>MARRLPKPTLQGRLEADFPDSPLLPKFQELNQNNLPNDVFREAQRSYLVFLTSQFCYEEYVQRTFGVPRRQRAIDKRQRASVAGAGAHAHLGGSSATPVQQAQAAASAGTGALASSAPSTAVAQSATPSVSSSISSLRAATSGATAAASAAAAVDTGSGGGGQPHDTAPRGARKKQ[4x];>MKVQGSVDRRRLQRRIAGLLPPPARRLNISRGSEFTRDVRGLVEEHAQASSLSAAAVWRAGLLAPGEVAVAGGGSGGGSFSWSGWRPPVFGDFLIHASSFNNAEATGTPLFQFKQSDPFSGVDAVFTPLSLFILMNHGRGVAARVEAGGGLTRMANLLYDSPATLADLVPDFGRLVADRRFHNFITPVGPLVENIKSTYLNKITTVVHGPVVSKAIPRSTVKVTVPQEAFVDLDAWLSGGAGGGGGVCFVGGLGLQPCPADARLYVALTYEEAGPRFTFFQSSRGHCQIMNILRIYYSPSIMHRYAVVQPLHIEELTFGAVACLGTFSATDGWRRSAFNYRGSSLPVVEIDSFYSNVSDWEVIL[2x];>[4x]MDLKVVVSLSSRLYTDEIAKMQQRIGCILPLASTHGTQNVQGLGLGQVYSLETVPDYVSMYNYLSDCTLAVLDEVSVDSLILTKIVPGQTYAIKNKYQPFFQWHGTGSLSVMPPVFGREHATVKLESNDVDIVFPMVLPTPIAEEVLQKILLFNVYSRVVMQAPGNADMLDVHMHLGSVSYLGHHYELALPEVPGPLGLALLDNLSLYFCIMVTLLPRASMRLVRGLIRHEHHDLLNLFQEMVPDEIARIDLDDLSVADDLSRMRVMMTYLQSLASLFNLGPRLATAAYSQETLTATCWLR;>[2x]MSNGDWGQSQRTRGTGPVRGIRTMDVNAPGGGSGGSALRILGTASCNQAHCKFGRFAGIQCVSNCVLYLVKSFLAGRPLTSRPELDEVLDEGARLDALMRQSGILKGHEMAQLTDVPSSVVLRGGGRVHIYRSAEIFGLVLFPAQIANSAVVQSLAEVLHGSYNGVAQFILYICDIYAGAIIIETDGSFYLFDPHCQKDAAPGTPAHVRVSTYAHDILQYVGAPGAQYTCVHLYFLPEAFETEDPRIFMLEHYGVYDFYEANGSGFDLVGPELVSSDGEAAGTPGADSSPPVMLPFERRIIPYNLRPLPSRSFTSDSFPAARYSPAKTNSPPSSPASAAPASAAPASAAPASAAPASAAPASAAPASAAPASAAPASSPPLFIPIPGLGHTPGVPAPSTPPRASSGAAPQTPKRKKGLGKDSPHKKPTSGRRLPLSSTTDTEDDQLPRTHVPPHRPPSAARLPPPVIPIPHQSPPASPTPHPAPVSTIAPSVTPSPRLPLQIPIPLPQAAPSNPKIPLTTPSPSPTAAAAPTTTTLSPPPTQQQPPQSAAPAPSPLLPQQQPTPSAAPAPSPLLPQQQPPPSAARAPSPLPPQQQPLPSATPAPPPAQQLPPSATTLEPEKNHPPAADRAGTEISPSPPFGQQPSFGDDASGGSGLVRYLSDLEEPFLSMSDSEEAESDLASDIPTTEDEDMFEDEVFSNSLESGSSAPTSPITLDTARSQYYQTTFDIETPEMDFVPLESNIARIAGHTYQEQAIVYDPASNREVPEADALSMIDYLLVTVVLEQGLIRSRDRSSVLNLLEFLKDWSGHLQVPTLDLEQLLTSELNIQNLANMLSENKGRAGEFHKHLAAKLEACLPSLATKDAVRVDAGAKMLAEIPQLAESDDGKFDLEAARRRLTDLLSGGDQEAGEGGGEPEDNSIYRGPHVDVPLVLDDESWKRLLSLAEAARTAVARQQAGVDEEDVRFLALLTAIEYGAPPAASVPPFVHNVAVRSKNAALHVRRCTADIRDKVASAASDYLSYLEDPSLPTVMDFDDLLTHLRHTCQIIASLPLLNIRYTSIEWDYRELLYLGTALSDMSGIPWPLERVEEDDPSIAPLPEFETVAKKQKELETTRENEKRLRTILDDIEAMLGLAGVASAPGAPISPASPSATPANHDNPEATPPLADTAALTIPVIEKYIANAGSIVGAAKNPTYIRLRDTIQQIVRSKKYLMNILKSITFYTIDNYIASFEESIDHLYRDLPVLDPEVQDGIDRILDPMVSEALHTFEMGNRLTLEPARLVALQNFATHSTLKETAAAVNLLPGLLAVYDATITGQAPEDALRLLSGLQNQLSQTLIPGKLKKRFLSYLQKLKNNNNDQLRQKEVQAWRLEAEGFKPATEEQLEAFLDTAPNKELKRQYEKKLRQLMETGRKEKEKLREQEDKERQERRAREANEAWARIRKALGARPEPAPTSPDDWNTLLASLLPDNTDSAAAAAAAVARNTDILDSLTQILAAMLLGITRVRRERLRSLLVDDGGAAERMEAAEPGWFTDIETGPLARLDAWPATPAATAKEGGGGRGAEEAAGALFRARTAADAIRSALAQTRQALQSPDMKSAVVNTDLEAPYAEYERGLAGLLEKRRAAEAALTAIVSEYVDRTLPEATNDPGQANLPPPPTIPQATAPPRLASDSALWPKKPQLLTRRERDDLLQATGDFFSELLTEAEAAEVRALEEQVRESQTLMAKAHEMAASTRRGFHTALEAVLSRSRDEAPDDELRSLLPSPPKAPVQAPLEAALARAAAGNGSWPYRKSLAAAKWIRGICEAVRGLSEGALALAGGAGAWLNLAAAADGEIHELTRLLEVEGMAQNSMDGMEELRLALATLDPKRVAGGKETVADWKRRLSRLEAIIQEAQEESQLQGTLQDLVTQARGHTDPRQLKIVVEAARGLALGASAGSQYALLKDKLLRYASAKQSFLAFYETAQPTVFVKHPLTNNLPLLITISAPPTGWGNGAPTRRAQFLAAAGPAKYAGTLWLETESPCDPLNPAYVSADTQEPLNYIPVYHNFLEYVMPTVLENPEAFSLTPAGRPQAIGPPQDDQERRRRTLASVASARLSAAAADSYWDTWPDVESNAGELLREYVSAPKALMEDLADNPIVAMTLLAHASLIASRNHPPYPAPATDREVILLEQREMMALLVGTHPAYAAAFLGAPSFYAGLGLVSALARDGGLGDLLSDSVLTYRLVRSPASGRGGMPSTTRGSNDGEDARRLTRHRIAGPPTGFIFFQDAWEEMDTRAALWPHPEFLGLVHNQSTARARACMLLLARRCFAPEALQQLWHSLRPLEGPVAFQDYLRDFVKQAYTRGEELPRAEGLEVPRETPSSYGTVTGRALRNLMPYGTPITGPKRGSGDTIPVSVFEAAVAAAFLGRPLTLFVSSQYLFNLKTLGQVRVVAPLLYCDGHSEPFRSLVETISLNFLQDLDGYSESFEPEMSIFARQAVWLRELLTEARAAKPKEARPPTVAILANRKNIIWKCFTYRHNLPDVQFYFNAAGASRWPTDVLNPSFYEHEDPPLPVGYQLPPNPRNVQELFSGFPPRVGHGLVSGDGFQSADNTPASSDRLQQLGGGETDQGEKGSTTAESEASGPPSPQSPLLEKVAPGRPRDWLSPTSSPRDVTVTPGLAAPITLPGPRLMARPYFGAETRASESPDRSPGSSPRPWPKDSLELLPQPAPQQPPSSPWASEQGPIVYTLSPHSTPSTASGSQKKHTIQIPGLVPSQKPSYPPSAPYKPGQSTGGIAPTPSAASLTTFGLQPQDTQASSQDPPYGHSIMQREKKQQGGREEAAEIRPSATRLPTAVGLRPRAPVVAAGAAASATPAFDPGEAPSGFPIPQAPALGSGLAAPAHTPVGALAPRPQKTQAQRPQDAAALPTPTIKAVGARPVPKATGALAAGARPRGQPTAAPPSAASPPRVSLPVRSRQQQSPAIPLPPMHSGSEPGARPEVRLSQYRHAGPQTYTVRKEAPPSAASQLPKMPKCKDSMYYPPSGSARYPAPFQALSFSQSVASPAPSSDQTTLLWNTPSVVTQFLSIEDIIREVVTGGSTSGDLVVPSGSPSSLSTAAPEQDLRYSLTLSQASRVLSRFVSQLRRKLERSTHRLIADLERLKFLYL;> MDVHIDNQVLSGLGTPLLVHLFVPDTVMAELCPNRVPNCEGAWCQTLFSDRTGLTRVCRVFAARGMLPGRPSHRGTFTSVPVYCDEGLPELYNPFHVAALRFYDEGGLVGELQIYYLSLFEGAKRALTDGHLIREASGVQESAAAMQPIPIDPGPPGGAGIEHMPVAAAQVEHPKTYDLKQILLEITQEENRGEQRLGHAGSPALCLGLRLRAGAETKAAAETSVSKHHPALENPSNIRGSAGGEGGGGRAGTGGTVGVGSGALSRVPVSFSKTRRAIRESRALVRGIAHIFSPHALYVVTYPELSAQGRLHRMTAVTHASPATDLAEVSILGAPEREFRFLISVALRISASFREKLAMQAWTAQQEIPVVIPTSYSRIYKNSDLIREAFFTVQTRVSWESCWVKATISNAPKTPDACLWIDSHPLYEEGASAWGKVIDSRPPGGLVGAASQLVALGTDGHCVHLATTSDGQAFLVLPGGFVIKGQLALTPEERGYILARHGIRREQ;>MALSGHVLIDPARLPRDTGPELMWAPSLRNSLRVSPEALELAEREAERARSERWDRCAQVLKNRLLRVELDGIMRDHLARAEEIRQDLDAVVAFSDGLESMQVRSPSTGGRSAPAPPSPSPAQPFTRLTGNAQYAVSISPTDPPLMVAGSLAQTLLGNLYGNINQWVPSFGPWYRTMSANAMQRRVFPKQLRGNLNFTNSVSLKLMTEVVAVLEGTTQDFFSDVRHLPDLQAALILSVAYLLLQGGSSHQQRPLPASREELLELGPESLEKIIADLKAKSPGGNFMILTSGNKEARQSIAPLNRQAAYPPGTFADNKIYNLFVGAGLLPTTAALNVPGAAGRDRDLVYRIANQIFGEDVPPFSSHQWNLRVGLAALEALMLVYTLCETANLAEAATRRLHLSSLLPQAMQRRKPAMASAGMPGAYPVQTLFRHGELFRFIWAHYVRPTVAADPQASISSLFPGLVLLALELKLMDGQAPSHYAINLTGQKFDTLFEIINQKLLFHDPAAMLAARTQLRLAFEDGVGVALGRPSPMLAAREILERQFSASDDYDRLYFLTLGYLASPVAPS[2x];>MASNEGVENRPFPYLTVDADLLSNLRQSAAEGLFHSFDLLVGKDAREAGIKFEVLLGVYTNAIQYVRFLETALAVSCVNTEFKDLSRMIDGKIQFRISVPTIAHGDGRRPSKQRTFIVVKNCHKHHISTEMELSMLDLEILHSIPETPVEYAEYVGAVKTVASALQFGVDALERGLINTVLSVKLRHAPPMFILQTLADPTFTERGFSKTVKSDLIAMFKRHLLEHSFFLDRAENMGSGFSQYVRSRLSEMVAAVSGESVLKGVSTYTTAKGGEPVGGVFIVTDNVLRQLLTFLGEEADNQIMGPSSYASFVVRGENLVTAVSYGRVMRTFEHFMARIVDSPEKAGSTKSDLPAVAAGVEDQPRVPISAAVIKLGNHAVAVESLQKMYNDTQSPYPLNRRMQYSYYFPVGLFMPNPKYTTSAAIKMLDNPTQQLPVEAWIVNKNNLLLAFNLQNALKVLCHPRLHTPAHTLNSLNAAPAPRDRRETYSLQHRRPNHMNVLVIVDEFYDNKYAAPVTDIALKCGLPTEDFLHPSNYDLLRLELHPLYDIYIGRDAGERARHRAVHRLMVGNLPTPLAPAAFQEARGQQFETATSLAHVVDQAVIETVQDTAYDTAYPAFFYVVEAMIHGFEEKFVMNVPLVSLCINTYWERSGRLAFVNSFSMIKFICRHLGNNAISKEAYSMYRKIYGELIALEQALMRLAGSDVVGDESVGQYVCALLDPNLLPPVAYTDIFTHLLTVSDRAPQIIIGNEVYADTLAAPQFIERVGNMDEMAAQFVALYGYRVNGDHDHDFRLHLGPYVDEGHADVLEKIFYYVFLPTCTNAHMCGLGVDFQHVAQTLAYNGPAFSHHFTRDEDILDNLENGTLRDLLEISDLRPTVGMIRDLSASFMTCPTFTRAVRVSVDNDVTQQLAPNPADKRTEQTVLVNGLVAFAFSERTRAVTQCLFHAIPFHMFYGDPRVAATMHQDVATFVMRNPQQRAVEAFNRPEQLFAEYREWHRSPMGKYAAECLPSLVSISGMTAMHIKMSPMAYIAQAKLKIHPGVAMTVVRTDEILSENILFSSRASTSMFIGTPNVSRREARVDAVTFEVHHEMASIDTGLSYSSTMTPARVAAITTDMGIHTQDFFSVFPAEAFGNQQVNDYIKAKVGAQRNGTLLRDPRTYLAGMTNVNGAPGLCHGQQATCEIIVTPVTADVAYFQKSNSPRGRAACVVSCENYNQEVAEGLIYDHSRPDAAYEYRSTVNPWASQLGSLGDIMYNSSYRQTAVPGLYSPCRAFFNKEELLRNNRGLYNMVNEYSQRLGGHPATSNTEVQFVVIAGTDVFLEQPCSFLQEAFPALSASSRALIDEFMSVKQTHAPIHYGHYIIEEVAPVRRILKFGNKVVF[4x]

Epstein-Bar virus (EBV), a member of the subfamily gammaherpesviruses that also includes the Kaposi Sarcoma-associated herpesvirus (KSHV),2,3 is the first identified oncovirus. Similar to other members of the family herpesviridae, EBV has a characteristic three-layer configuration: the outer lipid bilayer envelope containing viral glycoproteins responsible for host recognizing and membrane fusion, the inner pseudo-icosahedral nucleocapsid enclosing a 172-kb double-strand DNA (dsDNA) genome and the middle pleomorphic tegument compartment fulfilled with 20–40 different viral proteins. All herpesvirus capsid shell consists of 4 abundant proteins: the major capsid proteins (MCP) constituting the basic capsid skeleton through forming 150 hexons and 11 pentons, the small capsid proteins (SCP) binding to the tops of hexon MCPs or both hexon and penton MCPs, and the Tri1 and Tri2 forming the heterotrimeric triplexes to plug the large holes on the capsid floor. Once the viral dsDNA genome enters the procapsid shell through the portal that is located at a unique 5-fold vertex of the icosahedral capsid, the viral nucleocapsid is joined by the capsid-associated tegument complexes (CATCs).

By symmetry relaxation and localized classification, we sequentially resolved the structures of the C5 portal vertex, the C12 portal, the C1 portal vertex and the asymmetric capsid at resolutions of 4.2 Å, 4.8 Å, 5.5 Å and 7.5 Å, respectively, which enable us to build atomic models for the portal protein BBRF1 and the CATC proteins of BVRF1, BPLF1 and BGLF. Similar to that in KSHV,22 we also observed a turret-like density located between the C12 clip domain and the portal cap. Based on the agreement between the turret structure that is rich in helix-like densities and the secondary structure prediction of BBRF1, we tentatively assigned the turret to the unmodeled region of BBRF1’s clip domain. By docking the atomic models of the periportal capsid proteins and dodecameric portal into the C1 reconstruction of the portal vertex, we identified two portal regions involved in interactions with capsid proteins. The first one is the clip turret, which interacts with the trunk domains of five sets of Ta tri1 molecules. The second region is the portal wing, which interacts with capsid floor elements, including five sets of the spine helix in the P6 Johnson-fold, the β-barrel in the P1 Johnson-fold and the N-anchor of the periportal Ta. The C1 reconstruction of our portal vertex revealed CATC densities are as strong as those of the surrounding capsid proteins, indicating full occupancy of the five CATC registers surrounding the portal. The helix domains of the BVRF1 molecules and the two BPLF1 C-terminal regions form a helix bundle lying on the BGLF1 molecule. Each CATC binds both triplexes Ta and Tc.> MSVVGLDVGSQSCYIAVARAGGIETIANEFSDRCTPSVISFGSKNRTIGVAAKNQQITHANNTVSNFKRFHGRAFNDPFIQKEKENLSYDLVPLKNGGVGIKVMYMGEEHLFSVEQITAMLLTKLKETAENSLKKPVTDCVISVPSFFTDAERRSVLDAAQIVGLNCLRLMNDMTAVALNYGIYKQDLPSLDEKPRIVVFVDMGHSAFQVSACAFNKGKLKVLGTAFDPFLGGKNFDEKLVEHFCAEFKTKYKLDAKSKIRALLRLYQECEKLKKLMSSNSTDLPLNIECFMNDKDVSGKMNRSQFEELCAELLQKIEVPLYSLLEQTHLKVEDVSAVEIVGGATRIPA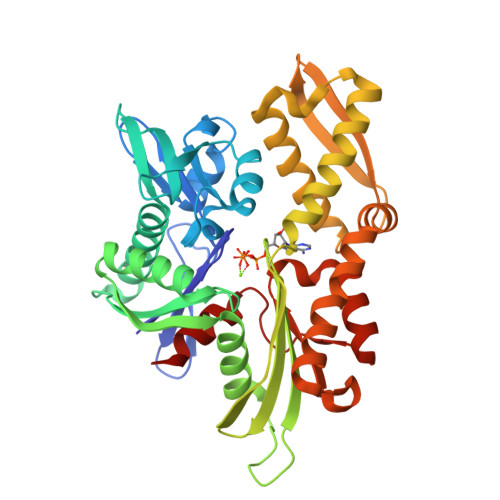VKERIAKFFGKDISTTLNADEAVARGCALQCS>MLGLKTSIIGRRVIYFQEITSTNEFAKTSYLEEGTVIVADKQTMGHGRLNAKWESPEGGLWLSIVLSPKVPQKDLPKIVFLGAVGVVETLKEFSIDGRIKWPNDVLVNYKKIAGVLVEGKGDKIVLGIGLNVNNKVPNGATSMKLELGSEVPLLSVFRSLITNLDR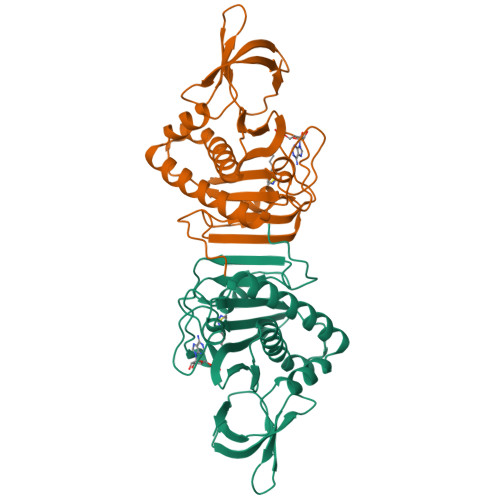LYLNFLKNPMDILNLVRDNMILGVRVKILGDGSFEGIAEDIDDFGRLIIRLDSGEVKKVIYGDVSLRFL[2x]>MKLKTTLFGNVYQFKDVKEVLAKANELRSGDVLAGVAAASSQERVAAKQVLSEMTVADIRNNPVIAYEDDCVTRLIQDDVNETAYNQIKNWSISELREYVLSDETSVDDIAFTRKGLTSEVVAAVAKICSNADLIYGAKKMPVIKKANTTIGIPGTFSARLQPNDTRDDVQSIAAQIYEGLSFGVGDAVIGVNPVTDDVENLSRVLDTIYGVIDKFNIPTQGCVLAHVTTQIEAIRRGAPGGLIFQSICGSEKGLKEFGVELAMLDEARAVGAEFNRIAGENCLYFETGQGSALSAGANFGADQVTMEARNYGLARHYDPFIVNTVVGFIGPEYLYNDRQIIRAGLEDHFMGKLSGISMGCDCCYTNHADADQNLNENLMILLATAGCNYIMGMPLGDDIMLNYQTT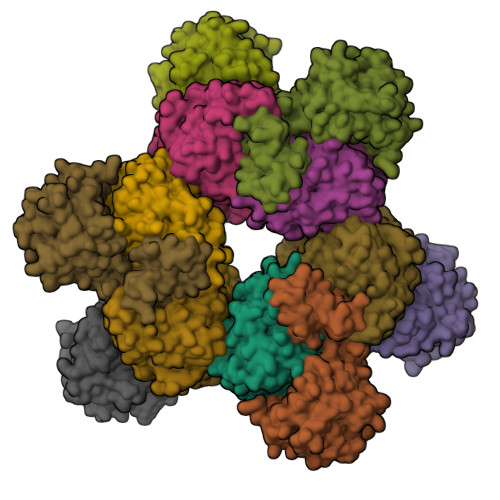AFHDTATVRQLLNLRPSPEFERWLESMGIMANGRLTKRAGDPSLFF[2x];>MDQKQIEEIVRSVMASMGQAAPAPSEAKCATTNCAAPVTSESCALDLGSAEAKAWIGVENPHRADVLTELRRSTVARVCTGRAGPRPRTQALLRFLADHSRSKDTVLKEVPEEWVKAQGLLEVRSEISDKNLYLTRPDMGRRLCAEAVEALKAQCVANPDVQVVISDGLSTDAITVNYEEILPPLMAGLKQAGLKVGTPFFVRYGRVKIEDQIGEILGAKVVILLVGERPGLGQSESLSCYAVYSPRMATTVEADRTCISNIHQGGTPPVEAAAVIVDLAKRMLEQKASGINMTR[2x]> MFDIALYEPEIAPNTGNIIRLCANCGANLHLIEPLGFDLEEKKVRRAGLDYHDLARVTRHKNYQAFLDYLEQRGEYRIFACTTKTTGHHVDAQYRQGDVLLFGPETRGLPMEVIESLPMSQRIRIPMMPDARSLNLSNAVAIIAFEAWRQLGFQGAKGHH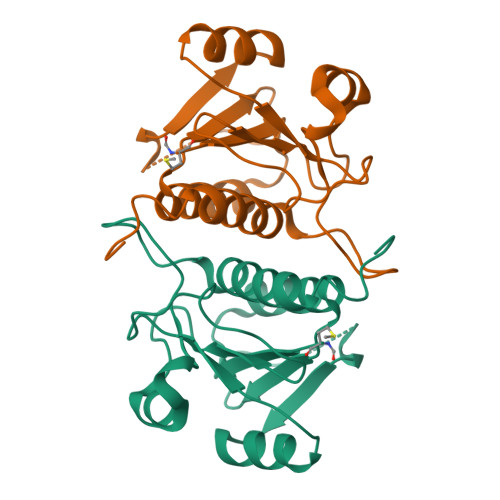HHHHG>SAMKPTAGPTTNADLTSAPPHDIFISHAWEDKADFVEALAHTLRAAGAEVWYDDFSLRPGDSLRRSIDKGLGSSRFGIVVLSTHFFKKEWPQKELDGLFQLESSGRSRILPIW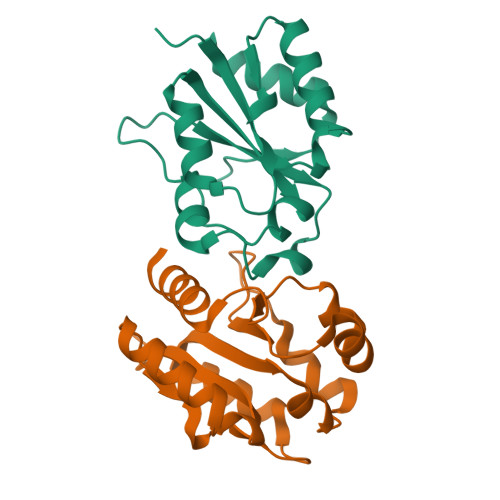HKVSKDEVASFSPTMADKLAFNTSTKSVDEIVADLMAIIRD[4x]> MGHHHHHHHHHHSSGHIDDDDKHMGSMAELKYISGFGNECSSEDPRCPGSLPEGQNNPQVCPYNLYAEQLSGSAFTCPRSTNKRSWLYRILPSVSHKPFESIDEGHVTHNWDEVDPDPNQLRWKPFEIPKASQKKVDFVSGLHTLCGAGDIKSNNGLAIHIFLCNTSMENRCFYNSDGDFLIVPQKGNLLIYTEFGKMLVQPNEICVIQRGMRFSIDVFEETRGYILEVYGVHFELPDLGPIGANGLANPRDFLIPIAWYEDRQVPGGYTVINKYQGKLFAAKQDVSPFNVVAWHGNYTPYKYNLKNFMVINSVAFDHADPSIFTVLTAKSVRPGVAIADFVIFPPRWGVADKTFRPPYYHRNCMSEFMGLIRGHYEAKQGGFLPGGGS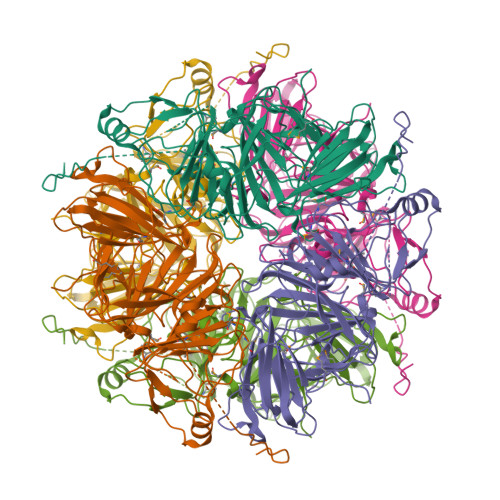LHSTMTPHGPDADCFEKASKVKLAPERIADGTMAFMFESSLSLAVTKWGLKASRCLDENYHKCWEPLKSHFTPNSRNPAEPN>MAGDTTITIVGNLTADPELRFTPSGAAVANFTVASTPRIYDRQTGEWKDGEALFLRCNIWREAAENVAESLTRGARVIVSGRLKQRSFETREGEKRTVIEVEVDEIGPSLRYATAKVNKASR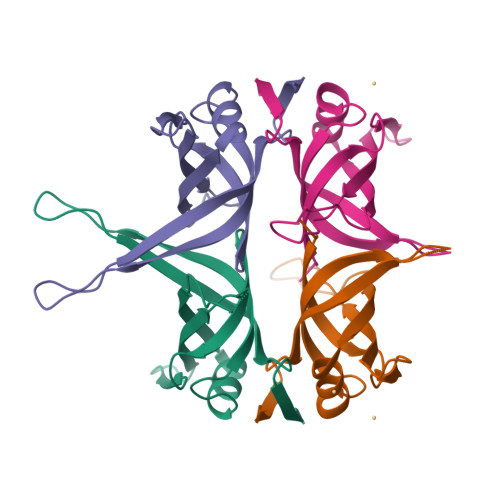SGGFGSGSRPAPAQTSSASGDDPWGSAPASGSFGGGDDEPPF[2x]>AHMNAGWVIGVDPDTSGALALLKPNQPPQVFDSPHLKVLVGKGVRKRLDAKAIVQLLKSFEAPIGTTVYVEQSTPYPQDGKQGWWSGGFGYGMWIGILVASGFSVIPVPSSAWKSEFQLTKERSNKDYSRQVASQL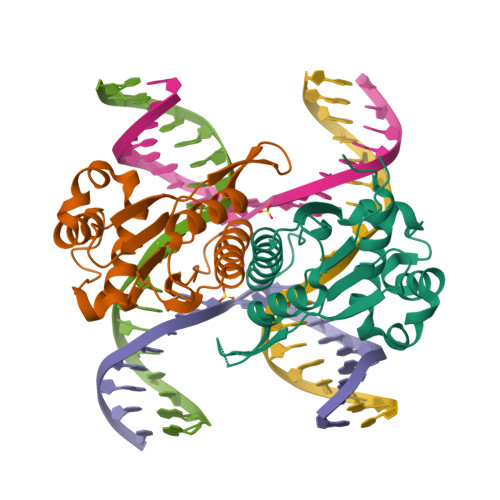FPSLSSLLKRKKDHGRAEALLIAAYGKGIKINSDS[2x]> GSHMASSTGVEITEGVTVTAKGNTEGNTADLAIDGDLSTYWESSNDYKWIEVDLGGIYELSKIEIFNKDEAVYKYNIYASEDGE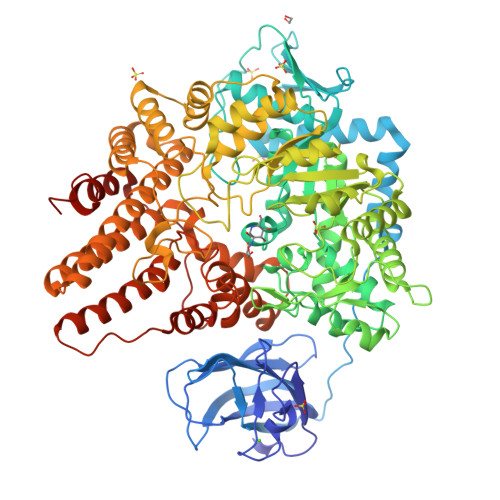NFNKIAYKNNDNVSDSNGNMHTIDNVRAGKIRIDVVQNSNSDRVNIAEINVFGKNTGESLPEVKKIATSNFSETPWATEYEKFNSDSAYANEKTLNEIKNLVGRVIGREFKDKFIFEIRDQLNGNDVFEVSDSGDGKVLIKGNNGVSLASGFNYYLKNYCNVSYNPIMGSNLKMPETMPSVGERVVIDTPYEHRYALNFCTYSYTMSFWDWDQYEEFLDWCAMNGVNLVLDIIGQEEVLRRTLNEFGYSDEEVKEFISGPAYFAWFYMQNMTGFGGPLPNDWFEQRAELGRKMHDRMQSFGINPVLQGYSGMVPRDFKEKNQEAQTISQGGWCGFDRPDMLKTYVNEGEADYFQKVADVFYEKQKEVFGDVTNFYGVDPFHEGGNTGDLDNGKIYEIIQNKMIEHDNDAVWVIQNWQGNPSNNKLEGLTKKDQAMVLDLFSEVSPDWNRLEERDLPWIWNMLHNFGGRMGMDAAPEKLATEIPKALANSEHMVGIGITPEAINTNPLAYELLFDMAWTRDQINFRTWTEDYIERRYGKTNKEILEAWNIILDTAYKKRNDYYQGAAESIINARPGFGIKSASTWGHSKIVYDKSEFEKAIEIFAKNYDEFKDSDAFLYDFADILKQLLANSAQEYYEVMCNAYNNGNGEKFKFVSGKFLELIKLQERVLSTRPEFLIGNWIEDARTMLKDSDDWTKDLFEFNARALVTTWGSRNNADGGGLKDYSNRQWSGLTEDYYYARWEKWINGLQAELDGGAKAPNIDWFKMEYDWVNKKSDTDKLYPTEASNENLGELAKIAMESYSVTNMDKILGENES>[2x]FNCNKREGPCSQR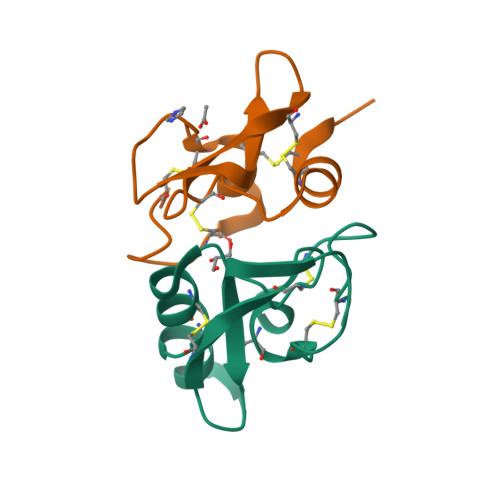SLCECDPNLQLGRHSDQLWHYNLRTNRCERGGYRDNCNSHSSSGACVMACERIHHHHHH>[4x]MSKFDVEQLLSELNQDEKISLLSAVDFWHTKKIERLGIPAVRVSDGPNGIRGTKFFDGVPSGCFPNGTGLASTFDRDLLETAGKLMAKESIAKNAAVILGPTTNMQRGPLGGRGFESFSEDPYLAGMATSSVVKGMQGEGIAATVKHFVCNDLEDQRFSSNSIVSERALREIYLEPFRLAVKHANPVCIMTAYNKVNGEHCSQSKKLLIDILRDEWKWDGMLMSDWFGTYTTAAAIKNGLDIEFPGPTRWRTRALVSHSLNSREQITTEDVDDRVRQVLKMIKFVVDNLEKTGIVENGPESTSNNTKETSDLLRKIAADSIVLLKNKNNILPLKKEDNIIVIGPNAKAKTSSGGGSASMNSYYVVSPYEGI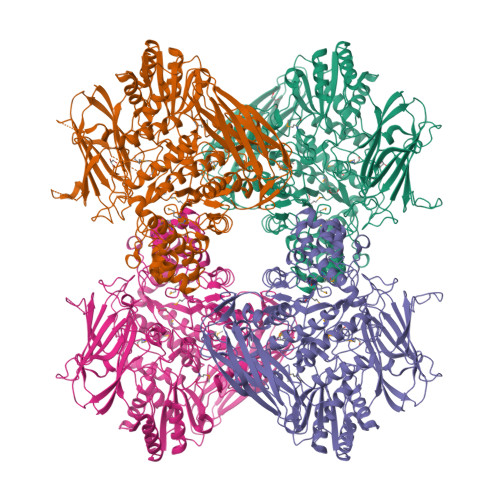VNKLGKEVDYTVGAYSHKSIGGLAESSLIDAAKPADAENSGLIAKFYSNPVEERSDDEEPFHVTKVNRSNVHLFDFKHEKVDPKNPYFFVTLTGQYVPQEDGDYIFSLQVYGSGLFYLNDELIIDQKHNQERGSFCFGAGTKERTKKLTLKKGQVYNVRVEYGSGPTSGLVGEFGAGGFQAGVIKAIDDDEEIRNAAELAAKHDKAVLIIGLNGEWETEGYDRENMDLPKRTNELVRAVLKANPNTVIVNQSGTPVEFPWLEDANALVQAWYGGNELGNAIADVLYGDVVPNGKLSLSWPFKLQDNPAFLNFKTEFGRVIYGEDIFVGYRYYEKLQRKVAFPFGYGLSYTTFELDISDFKVTDDKIAISVDVKNTGDKFAGSEVVQVYFSALNSKVSRPVKELKGFEKVHLEPGEKKTVNIDLELKDAISYFNEELGKWHVEAGEYLVSVGTSSDDILSVKEFKVEKELYWKGL There are three parts to the flagellar structure: the trans-membrane basal body that functions as the motor, the connecting rod and hook, and the flagellar filament that acts like a helical propeller. Our current understanding of supercoiling in bacterial flagellar filaments, referred to as polymorphic switching, is based upon the notion that protofilaments within the flagellar filament can exist in two discrete states, that differ slightly in length. The “short” state results from a protofilament having a right-handed inclination (the R-state), while the “long” state results from a protofilament having a left-handed inclination (the L-state). To reconstruct filaments at high resolution, all protofilaments must be “locked” into the same state, either L- or R-type, producing straightened filaments that lead to non-motile bacteria.

Next, we analyzed flagellar filaments from the Gram-negative bacterium Pseudomonas aeruginosa to compare with a Gram-negative species. Since the D0 and D1 domains of P. aeruginosa and S. enterica share a high degree of sequence identity (55%), we tested the conserved L- and R-type mutations characterized in S. enterica (G426A and A449V, respectively), which correspond to G420A and A443V in P. aeruginosa, respectively. We found that these mutations also generate straightened filaments in this organism. Filaments from these two FliC mutants of P. aeruginosa were sheared off the bacteria, concentrated, plunge-frozen and cryo-EM imaged. Each mutation results in L- and R-type straight filaments as expected, which suggests that the D0/D1 architecture is indeed conserved between P. aeruginosa and S. enterica. For both the L- and R-type P. aeruginosa filaments, we identified three pseudo layer-lines in the power spectra from the filaments, besides the 1-, 5-, 6- and 11-start layer-lines that are similar to B. subtilis, which correspond to non-helical perturbations. We obtained near-atomic resolution reconstructions for the D0 and D1 domains for both mutants: at 4.2 Å resolution for L-type filament G420A and at 4.3 Å resolution for R-type filament A443V based on FSC of the cryo-EM density map with the resulting filament model. That we could reach such a resolution for D0 and D1 confirms that the perturbation is entirely limited to the outer D2/D3 domains, as previously suggested from lower resolution studies of other bacteria. The three L-type subunits of B. subtilis and one L-type subunit of P. aeruginosa aligned very well in both D0 and D1 domains. From our structures, in P. aeruginosa the D3 domain extends along the 11-start and forms a dimer with the D2 domain of another subunit; while in S. enterica, the D3 domain extends from the filament and does not interact with other subunits.

>[41x]MALTVNTNIASLNTQRNLNASSNDLNTSLQRLTTGYRINSAKDDAAGLQISNRLSNQISGLNVATRNANDGISLAQTAEGALQQSTNILQRIRDLALQSANGSNSDADRAALQKEVAAQQAELTRISDTTTFGGRKLLDGSFGTTSFQVGSNAYETIDISLQNASASAIGSYQVGSNGAGTVASVAGTATASGIASGTVNLVGGGQVKNIAIAAGDSAKAIAEKMDGAIPNLSARARTVFTADVSGVTGGSLNFDVTVGSNTVSLAGVTSTQDLADQLNSNSSKLGITASINDKGVLTITSATGENVKFGAQTGTATAGQVAVKVQGSDGKFEAAAKNVVAAGTAATTTIVTGYVQLNSPTAYSVSGTGTQASQVFGNASAAQKSSVASVDISTADGAQNAIAVVDNALAAIDAQRADLAAVQNRFKNTIDNLTNISENATNARSRIKDTDFAAETAALSKNQVLQQAGTAILAQANQLPQAVLSLLR6-azanyl-9-[(2R,3R,4S,5R)-3,4-dihydroxy-5-(hydroxymethyl)oxolan-2-yl]-7H-purin-8-one 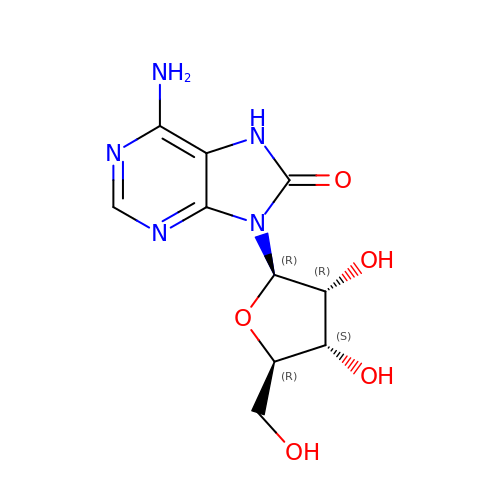| C10 H13 N5 O5 | UEHOMUNTZPIBIL-UUOKFMHZSA-N6-azanyl-1-[2-(azetidin-3-yl)ethyl]-2-cycloheptyl-4-ethoxy-pyrazolo[3,4-d]pyrimidin-3-one 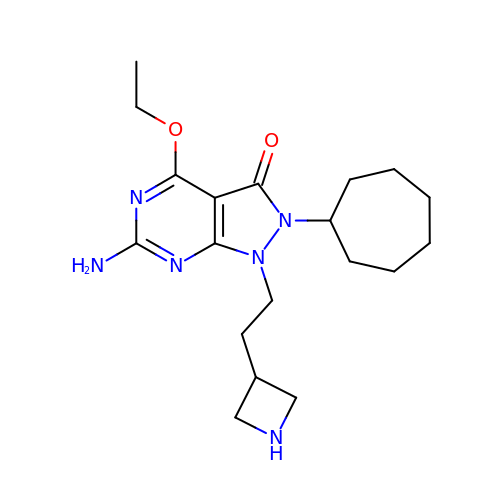| C19 H30 N6 O2 | KMGTYIPXRJPIEX-UHFFFAOYSA-N> SAERRALKIGVNGIPVTLEPINAISNVGPRIVNQIFDTLVVRDFFSNGAPGNGINLMPSLAESWERIDDKSVRFKLRQKVMFHDGVEMTADDVAYTFSSERLWGPDAIKVIPLGGSYALDFDEPVVEDKYTVVIRTKTPTPLTESYMASWMGRIVPKAYYKTLGTAAFGNKPVGTGPYKFVEFVANDRVVIEANDAYWGLKPTASKITYQLVAEPATRVAGLISGEYDIVTTLTPDDMALINSYPDLETRGNIVENFHMFTFNMNQPVFQS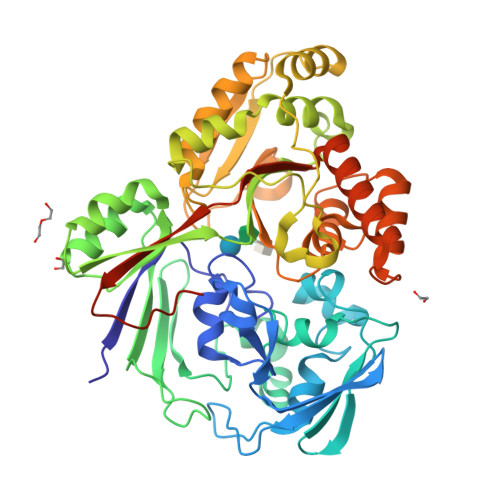KPLRRALALAVNRPLIVQSLWMNKATIPNGFNFPNYGKTFDPNRRAMEYNIEEAKRLVKESGYDGTPITYHTMGNYYANAVPALMMMIEMWKQIGVTVVPKVYAPGGAPKDQDSYMRNWSNGQWMTDAWATMICEFGPKGQVQKRWGWKAPAEFNDLCTKVSQIPDSKERFDAFNRLRDIFEEEAPAVILYQPFDVYAARKDVHWRPISFEMMEFRNNLAFGHHHHHH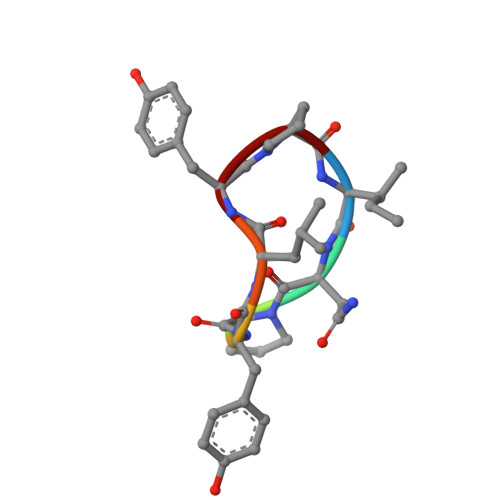> INPYLYP> LGTNYLLSGQTLDREGHLKNGDFDLVMQDDCNLVLYNGNWQSNTANKGRDCKLTLTDYGELVIKNG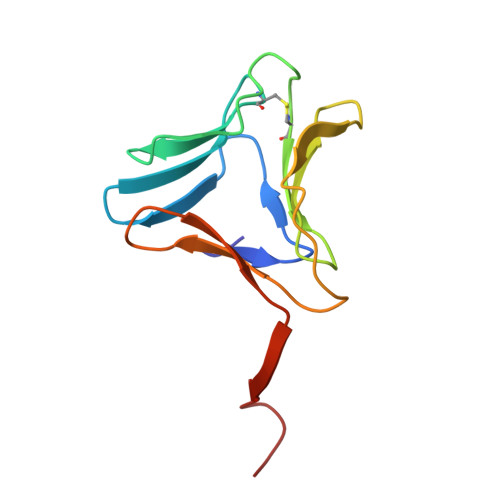DGSTVWRSRAQSVKGNYAAVVHPDGRLVVFGPSVFKIDPWVPG>[2x]MMITLDHVTKQYKSSARPALDDINVKIDKGEFVFLIGPSGSGKSTFMRLLL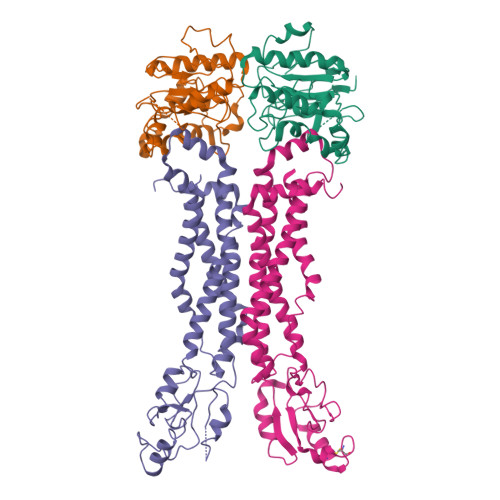AAETPTSGDVRVSKFHVNKLRGRHVPKLRQVIGCVFQDFRLLQQKTVYDNVAFALEVIGKRTDAINRVVPEVLETVGLSGKANRLPDELSGGEQQRVAIARAFVNRPLVLLADEPTGNLDPETSRDIMDLLERINRTGTTVLMATHDHHIVDSMRQRVVELSLGRLVRDEQRGVYGMDR;>MRFGFLLNEVLTGFRRNVTMTIAMILTTAISVGLFGGGMLVVRLADSSRAIYLDRVESQVFLTEDVSANDSSCDTTACKALREKIETRSDVKAVRFLNRQQAYDDAIRKFPQFKDVAGKDSFPASFIVKLENPEQHKDFDTAMKGQPGVLDVLNQKELIDRLFAVLDGLSNAAFAVALVQAIGAILLIANMVQVAAYTRRTEIGIMRLVGASRWYTQLPFLVEAMLAATMGVGIAVAGLMVVRALFLENALNQFYQANLIAKVDYADILFITPWLLLLGVAMSGLTAYLTLRLYVRR[2x]>KKTSGNQDEILVIRKGWLTINNIGIMKGGSKEYWFVLTAENLSWYKDDEEKEKKYMLSVDNLKLRDVEKGFMSSKHIFALFNTEQRNVYKDYRQLELACE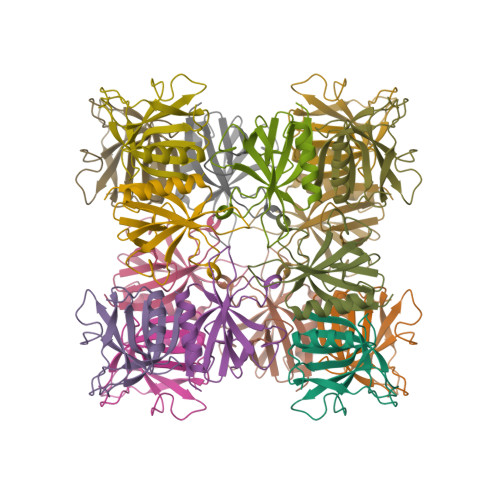TQEEVDSWKASFLRAGVYPERV[2x]>[60x]MEE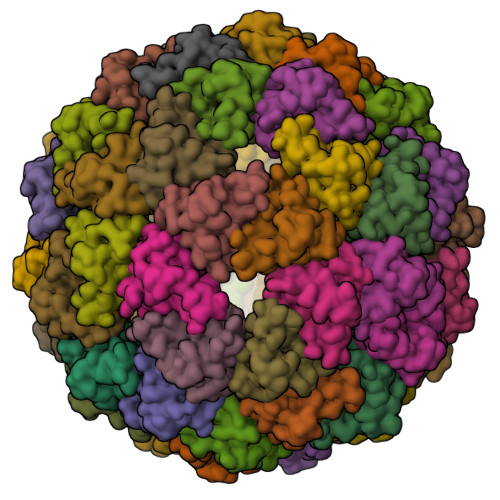ERRRHLAAAEARFLLELGRPDEVLRLLERLLEEGDPALFAALRELLESGDPLARLIAETVFRRL>IVDTCSLASPASVCRTKHLHLRCSVDFTRRTLTGTAALTVQSQEDNLRSLVLDTKDLTIEKVVINGQEVKYALGERQSYKGSPMEISLPIALSKNQEIVIEISFETSPKSSALQWLTPEQTSGKEHPYLFSQCQAIHCRAILPCQDTPSVKLTYTAEVSVPKELVALMSAIRDGETPDPEDPSRKIYKFIQKVPIPCYLIALVVGALESRQIGPRTLVWSEKEQVEKSAYEFSETESMLKIAEDLGGPYVWGQYDLLVLPPSFPYGGMENPCLTFVTPTLLAGDKSLSNVIAHEISHSWTGNLVTNKTWDHFWLNEGHTVYLERHICGRLFGEKFRHFNALGGWGELQNSVKTFGETHPFTKLVVDLTDIDPDVAYSSVPYEKGFALLFYLEQLLGGPEIFLGFLKAYVEKFSYKSITTDDWKDFLYSYFKDKVDVLNQVDWNAWLYSPGLPPIKPNYDMTLTNACIALSQRWITAKEDDLNSFNATDLKDLSSHQLNEFLAQTLQRAPLPLGHIKRMQEVYNFNAINNSEIRFRWLRLCIQSKWEDAIPLALKMATEQGRMKFTRPLFKDLAAFDKSHDQAVRTYQEHKASMHPVTAM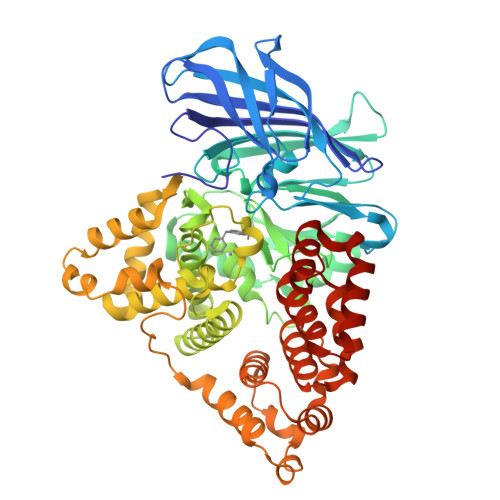LVGKDLKVD[3x]Human α‐l‐iduronidase (IDUA), which belongs to the GH39 family in the Carbohydrate Active EnZyme (CAZy) classification, hydrolyzes terminal non‐reducing α‐l‐iduronic acid residues in glycoaminoglycans (GAGs), including dermatan sulfate (DS) and heparan sulfate (HS), through a two‐step Koshland double‐displacement mechanism. The active site of the enzyme contains a carboxylic acid/carboxylate pair that acts as an acid/base (Glu188) and a nucleophilic (Glu299) catalyst. Mutations in the gene encoding IDUA may result in mucopolysaccharidosis type I (MPS I), which is a rare autosomal inherited recessive disease that leads to toxic accumulation of HS and DS. The structures of IDUA when complexed with the inhibitors in a non‐covalent transition state mimicking form and a covalent enzyme‐bound form provide insights into its conformational itinerary.

In an attempt to fully define the conformational inhibition of compounds 1–3, raIDUA crystals were soaked with the ABPs for shorter durations. Data collected to 2.39 Å resolution on a crystal soaked with ABP 3 for 45 min revealed electron density in the active site of raIDUA consistent with the unreacted cyclophellitol aziridine 3. A methyl group on the cyclophellitol aziridine was visible, but the rest of the R group was not evident and presumably disordered. Interestingly, the pseudo‐glycoside was observed in a 2, 5B conformation, which is the predicted transition state for GH39 α‐l‐iduronisase. The majority of the interactions with active site residues were the same as those described for the covalent complex with raIDUA, although a shift in position of the glycoside indicated that the carboxylate group additionally interacted with Lys264. The hydroxyl group at C2 forms a hydrogen bond with the nucleophile Oϵ2 of Glu299, but at a surprisingly short distance of 2.4 Å, suggesting a tight interaction. This close proximity results in a distance between the pseudo‐anomeric carbon and Oϵ1 of only 2.9 Å. Superimposition of the main‐chain atoms for the two complexes revealed a shift in the position of the cyclophellitol aziridine to accommodate formation of the covalent bond. This engendered movement of between 0.2 and 0.4 Å at C5, C4, and C3, 0.5 Å at C2, 0.6 Å at the carbon at the position of the endocyclic oxygen, and 1.1 Å at the pseudo‐anomeric carbon.

> EAPHLVQVDAARALWPLRRFWRSTGFCPPLPHSQADPYVLSWDQQLNLAYVGAVPHRGIKQVRTHWLLELVTTRGSTGRGLSYNFTHLDGYLDLLRENQLLPGFELMGSASGHFTDFEDKQQVFEWKDLVSSLARRYIGRYGLAHVSKWNFETWNEPDHHDFDNVSMTMQGFLNYYDACSEGLRAASPALRLGGPGDSFHTPPRSPLSWGLLRHCHDGTNFFTGEAGVRLDYISLHRKGARSSISILEQEKVVAQQIRQLFPKFADTPIYNDEADPLVGWSLPQPWRADVTYAAMVVKVIAQHQNLLLANTTSAFPYALLSNDNAFLSYHPHPFAQRTLTARFQVNNTRPPHVQLLRKPVLTAMGLLALLDEEQLWAEVSQAGTVLDSNHTVGVLASAHRPQGPADAWRAAVLIYASDDTRAHPNRSVAVTLRLRGVPPGPGLVYVTRYLDNGLCSPDGEWRRLGRPVFPTAEQFRRMRAAEDPVAAAPRPLPAGGRLTLRPALRLPSLLLVHVCARPEKPPGQVTRLRALPLTQGQLVLVWSDEHVGSKCLWTYEIQFSQDGKAYTPVSRKPSTFNLFVFSPDTGAVSGSYRVRALDYWARPGPFSDPVPYLEVPVPRGPPSPGNP;> EAPHLVQVDAARALWPLRRFWRSTGFCPPLPHSQADPYVLSWDQQLNLAYVGAVPHRGIKQVRTHWLLELVTTRGSTGQGLSYNFTHLDGYLDLLRENQLLPGFELMGSASGHFTDFEDKQQVFEWKDLVSSLARRYIGRYGLAHVSKWNFETWNEPDHHDFDNVSMTMQGFLNYYDACSEGLRAASPALRLGGPGDSFHTPPRSPLSWGLLRHCHDGTNFFTGEAGVRLDYISLHRKGARSSISILEQEKVVAQQIRQLFPKFADTPIYNDEADPLVGWSLPQPWRADVTYAAMVVKVIAQHQNLLLANTTSAFPYALLSNDNAFLSYHPHPFAQRTLTARFQVNNTRPPHVQLLRKPVLTAMGLLALLDEEQLWAEVSQAGTVLDSNHTVGVLASAHRPQGPADAWRAAVLIYASDDTRAHPNRSVAVTLRLRGVPPGPGLVYVTRYLDNGLCSPDGEWRRLGRPVFPTAEQFRRMRAAEDPVAAAPRPLPAGGRLTLRPALRLPSLLLVHVCARPEKPPGQVTRLRALPLTQGQLVLVWSDEHVGSKCLWTYEIQFSQDGKAYTPVSRKPSTFNLFVFSPDTGAVSGSYRVRALDYWARPGPFSDPVPYLEVPVPRGPPSPGNP> MMNRFRKWLYKPKRSDPQLLARFYYADEELNQVAAELDSLDGRKDPQRCTLLVSQFRSCQDNVLNIINQIMDECIPQDRAPRDFCVKFPEEIRHDNLAGQLWFGAECLAAGSIIMNRELESMAMRPLAKELTRSLEDVRGALRDQALRDLNTYTEKMREALRHFDVLFAEF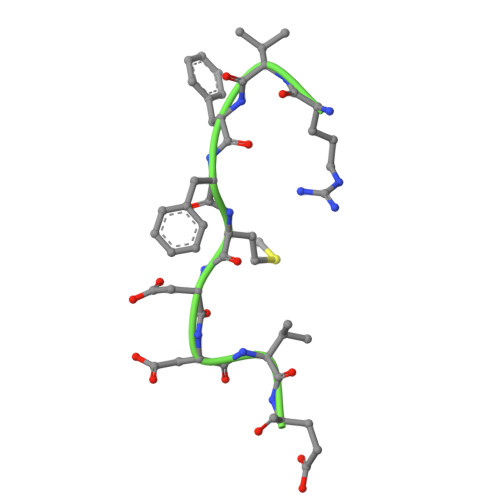ELSYVSAMVPVKSPREYYVQQEVIVLFCETVERALDFGYLTQDMIDDYEPALMFSIPRLAIVCGLVVYADGPLNLDRKVEDMSELFRPFHTLLRKIRDLLQTLTEEELHTLERNLCISQDVEFPIRADVQGPAALAPALSAPLPPEGPLSAKAKDPDAELACSMQYDDQELEQLSRMVHRAGDEMSSLLSPPIACQSPAHRPGAEGSPGGEASPGRPRLRSGSDEEERVFFMDDVEGTAEALARPESPAGPFGWAGSTWADPQEKGQGGPGGAAGISLPASEKEEDLSNNNLEAEGTDGASLAGTSSCSCLDSRLHLDGWEVGADDAETAEMIAHRTGGMKLSATVIFNPKSPTSLDSAVATQEAASEPVAEGMDGGPHKLSTGATNCLLHSCVCCGSCGDSREDVVERLREKCSPGGVIGASYAAGLAKASDRAPERQEEAPPPSEDASNGREPKAPTSDKCLPHTSGSQVDTASGLQGEAGVAGQQEPEARELHAGSPSAHEAPQALSGSSSSTAGSCSSDKMGPEAAPAATHAAPQATREKIRSRFHGSHDLIHRLFVCISGVADQLQTNYASDLRSILKTLFEVMATKPETDDKEKLRKVTQTLRSAALEDCALCQETLSSSELAAKTRDGDFEDPPEWVPDEACGFCTACKAPFTVIRRKHHCRSCGKIFCSRCSSHSAPLPRYGQVKPVRVCTHCYMFHVTPFYSDKAGL>[2x]MGRDKKNTALLDIARDIGGDEAVEVVKALEKKGEATDEELAELTGV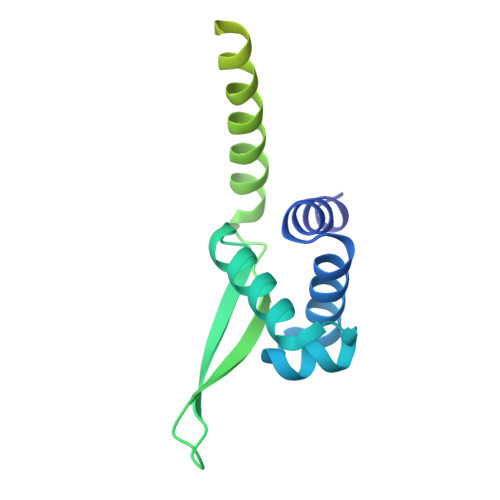RVNTVRKILYALYDAKLATFRRVRDDETGWYYYYWRIDTKRLPEVIRTRKLQELEKLKQMLQEETSETYYHCGTPGHPKLTFDEAFEYGFQCPICGEILYEYDNSKIIEELKKRIEELEIELGLRSPPKEEKPKKATRRKKSRSGKKKK> NVIQDLYLRELKDTKLAPSTLQDAEGNVKPWNPPQKPNLPELELQGPEALKAYTEQNVETAHVAKESEEGESEPIEEDWLVLDD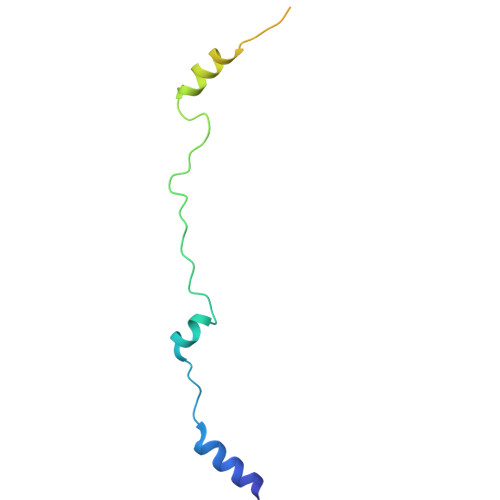AEETKESH3-[(2-methyl-6-phenylpyridin-4-yl)oxy]phenol 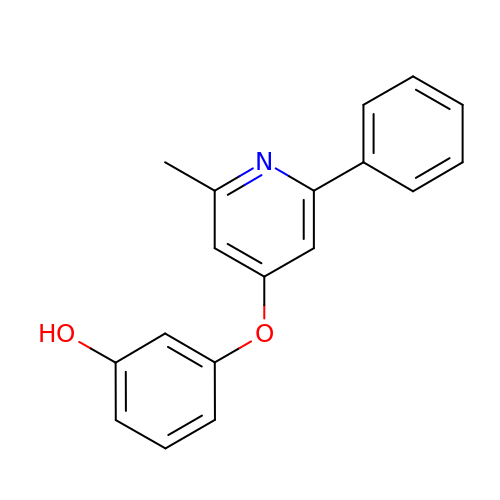| C18 H15 N O2 | SJHYRSDSTDNDIP-UHFFFAOYSA-N>MGPLPRTVELFYDVLSPYSWLGFEILCRYQNIWNINLQLRPSLITGIMKDSGNKPPGLLPRKGLYMANDLKLLRHHLQIPIHFPKDFLSVMLEKGSLSAMRFLTAVNLEHPEMLEKASRELWMRVWSRNEDITEPQSILAAAEKAGMSAEQAQGLLEKIATPKVKNQLKETTEAACRYGAFGLPITVAHVDGQTHMLFGSDRMELLAHLLGEKWMGP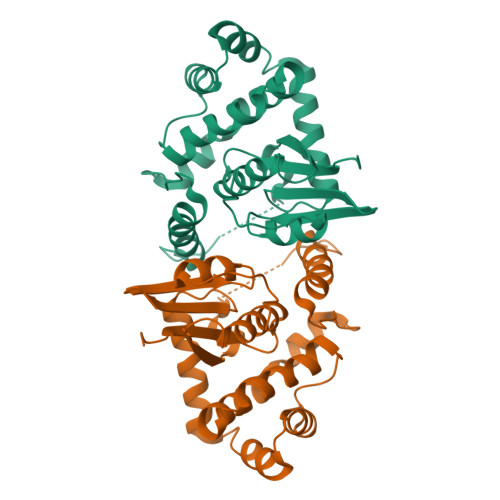IPPAVNARLLEHHHHHH[3x]> MRYFRPLSATAMTTVLLLAGTNVRAQPTEPTPASAHRPSISRGHYLAIAADCAACHTNGRDGQFLAGGYAISSPMGNIYSTNITPSKTHGIGNYTLEQFSKALRHGIRADGAQLYPAMPYDAYNRLTDEDVKSLYAYIMTEVKPVDAPSPKTQLPFPFSIRASLGIWKIAARIEGKPYVFDHTHNDDWNRGRYLVDELA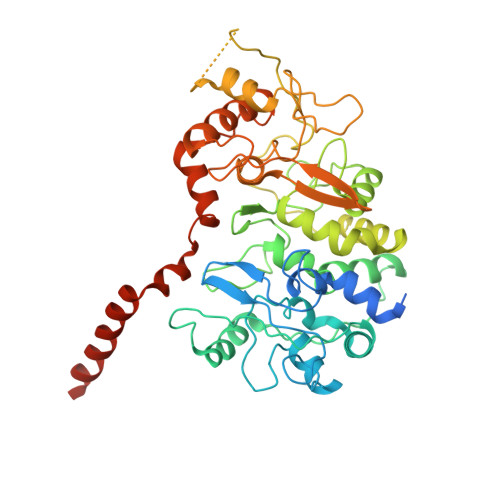HCGECHTPRNFLLAPNQSAYLAGADIGSWRAPNITNAPQSGIGSWSDQDLFQYLKTGKTAHARAAGPMAEAIEHSLQYLPDADISAIVTYLRSVPAKAESGQTVANFEHAGRPSSYSVANANSRRSNSTLTKTTDGAALYEAVCASCHQSDGKGSKDGYYPSLVGNTTTGQLNPNDLIASILYGVDRTTDNHEILMPAFGPDSLVQPLTDEQIATIADYVLSHFGNAQATVSADAVKQVRAGGKQVPLAKLASPGVMLLLGTGGILGAILVVAGLWWLISRRKKRSA> MVGLTTLFWLGAIGMLVGTLAFAWAGRDAGSGERRYYVTLVGISGIAAVAYVVMALGVGWVPVAERTVFAPRYIDWILTTPLIVYFLGLLAGLDSREFGIVITLNTVVMLAGFAGAMVPGIERYALFGMGAVAFLGLVYYLV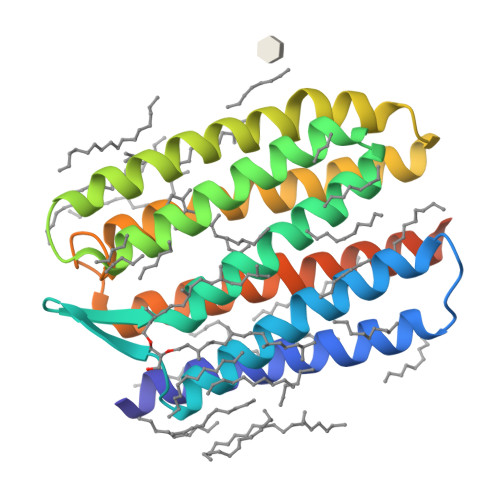GPMTESASQRSSGIKSLYVRLRNLTVILWAIYPFIWLLGPPGVALLTPTVDVALIVYLDLVTKVGFGFIALDAAATLRAEHGESLAGVDTDAPAVAD> LSKNVVAVNEELTDALAEEWKRRYEKEKEKNARLKGKVEDLEKERDFYFGKLRNIEL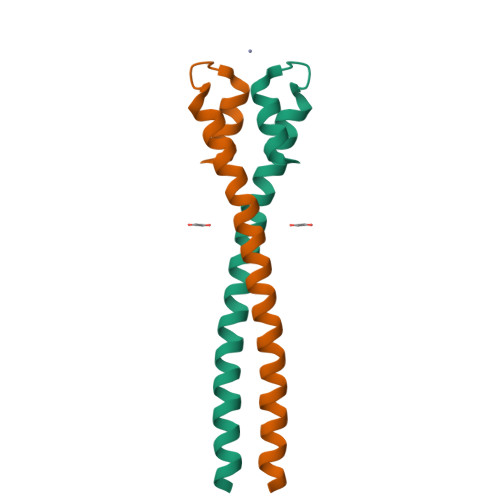ICQENEGENDPVLQRIVDILYATDEGFVIPD>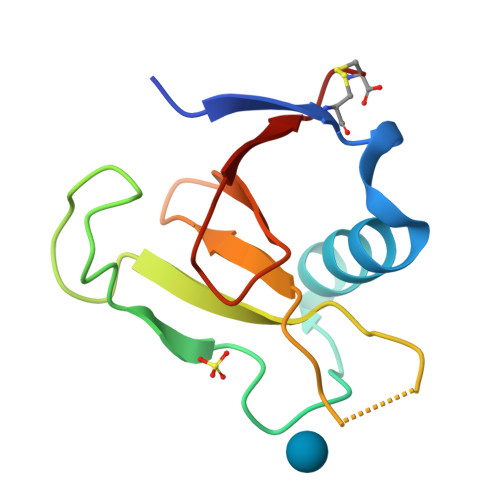ADPALADVCRTKLPSQAQDTLALIAKNGPYPYNRDGVVFENRESRLPKKGNGYYHEFTVVTPGSNDRGTRRVVTGGYGEQYWSPDHYATFQEIDPRC[3x]> MHHHHHHENLYFQTNPEALTVAATEVRRIRDRAIQSDAQVAPMTTAVRPPAADLVSEKAATFLVEYARKYRQTIAAAA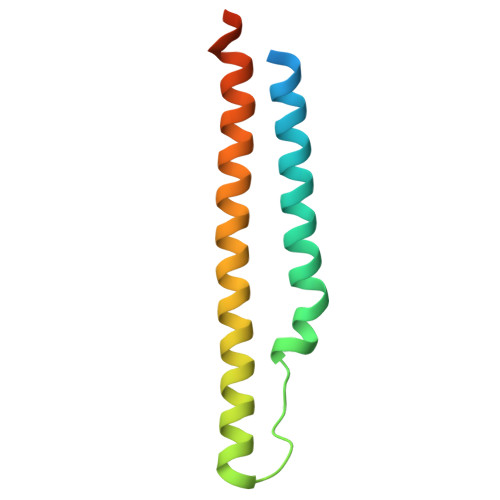VVLEEFAHALTTGADKYATAEADNIKTFS>QQFPQFHVKSGLQIKKNAIIDDYKVTSQVLGLGINGKVLQIFNKRTQEKFALKMLQDCPKARREVELHWRASQCPHIVRIVDVYENLYAGRKCLLIVMECLDGGELFSRIQDRGDQAFTEREASEIMKSIGEAIQYLHSINIAHRDVKPENLLYTSKRPNAILKLTDFGFAKETTSHNSLTTPCYTPYYVAPEVLGPEKYDKSCDMWSLGVIMYILLCGYPPFYSNHGLAISPGM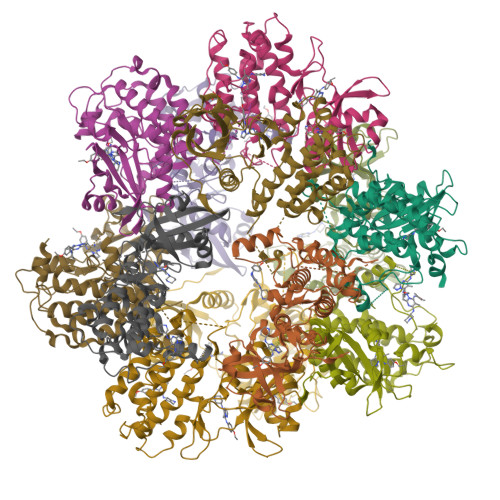KTRIRMGQYEFPNPEWSEVSEEVKMLIRNLLKTEPTQRMTITEFMNHPWIMQSTKVPQTPLHTSRVLKEDKERWEDVKEEMTSALATMR[12x]>[4x]MKNERIEKLQESWELDERWEGITRPYSAEDVIRLRGSIDIEHTLARRGAEKLWTSLHTEDYINALGALTGNQAMQQVKAGLKAIYLSGWQVAADANLSGHMYPDQSLYPANSVPAVVKRINQTLQRADQIQHMEGSDDTDYFV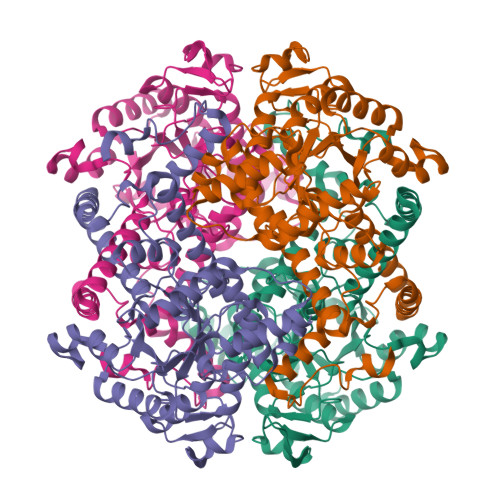PIVADAEAGFGGQLNVFELMKGMIEAGASGVHFEDQLSSEKKCGHLGGKVLLPTQTAVRNLISARLAADVMGVPTIIVARTDADAADLITSDIDPVDKAFITGERTPEGFYRTNAGLDQAIARGLAYAPYADLVWCETSEPNLEDAKRFADAIHKEHPGKLLAYNCSPSFNWKQKLDEKAIASFQKEIASYGYKFQFVTLAGFHSLNYGMFELARGYKERGMAAYSELQQAEFAAEKHGYSATRHQREVGTGYFDEVAQVITGGTSSTTALKGSTEEAQFTKLEHHHHHH> LKEIIASNPDDLTTELKRAFRPLTPHIAIDGNEIDALTILVNLTDKAKCKQKLRDEKWWASCINCVNYRQSHNPKFPDIRSEGVIRTQALGELPSFLLSSSKIPPYHWSYSHDSKYVNKSAFLTNEFCWDGEISCLGELLKDADHPLWNTLKKLGCSQKTCKAMAKQLADITLTTINVTLAPNYLTQISLPDSDTSYISLSPVASLSMQSHFHQRLQDENRHSAITRFSRTTNMGVTAMTCGGAFRMLKSGAKFSSPPHHRLNNGSFLVLPNIRVCGATALSSPVTVGIPSLTAFFGFVHAFERNINRTTSSFRVESFAICVHQLHVEKRGLTAEFVEKGDGTISAPATRDDW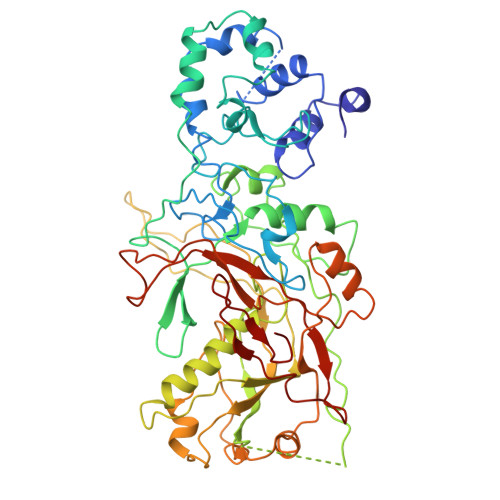QCDVVFSLILNTNFAQHIDQDTLVTSLPKRLARGSAKIAIDDFKHINSFSTLETAIESLPIEAGRWLSLYAQSNNNLSDLLAAMTEDHQLMASCVGYHLLEEPKDKPNSLRGYKHAIAECIIGLINSITFSSETDPNTIFWSLKNYQNYLVVQPRSIN> SDHSIEVTFRVKTQQVIIPEQNIRGNELPLRRWQMELLMLDATGKEVEPTILSKCIYHLHSSFKQPKRRLNSLPFFIKETGWG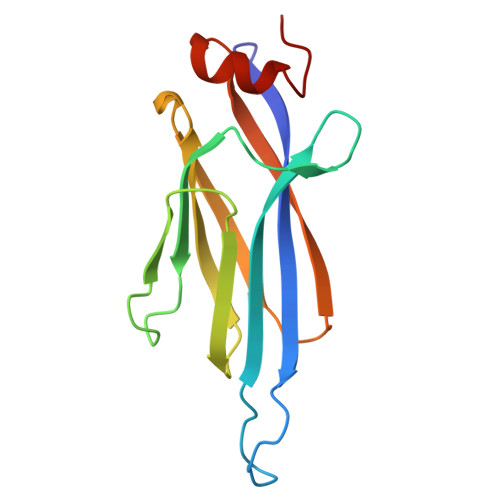EFNLKIECFFIGNAGKFSIEHDLTFEDDAYAVDYTVDVPHEFSHLNSELSKYFDLP2-[(4,4-difluoro-1-phenylcyclohexyl)amino]-N-hydroxypyrimidine-5-carboxamide 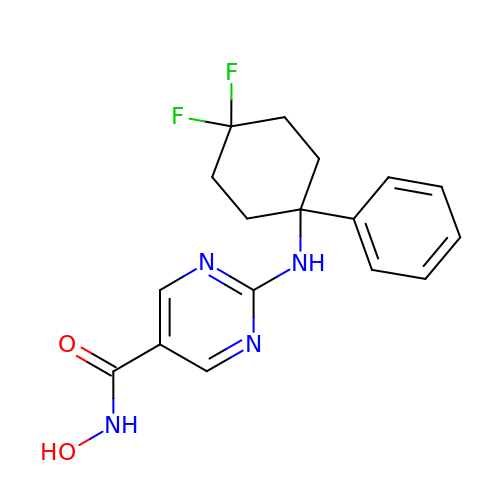| C17 H18 F2 N4 O2 | MRWCVKLVSWYIFO-UHFFFAOYSA-N4-hydroxyquinoline-3,8-dicarboxylic acid | C11 H7 N O5 | 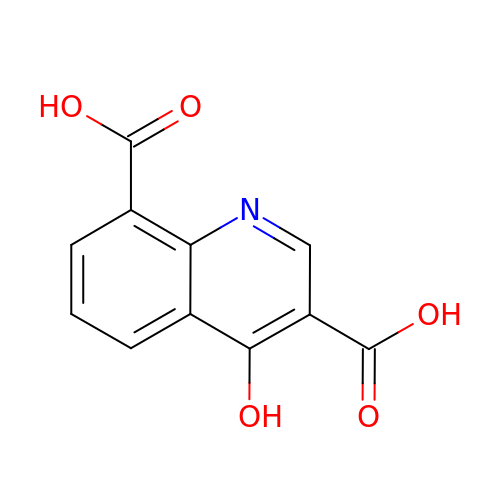YYLVBIBWUBXXRA-UHFFFAOYSA-N pyrimido[5,4-e][1,2,4]triazine-5,7(6H,8H)-dione | C5 H3 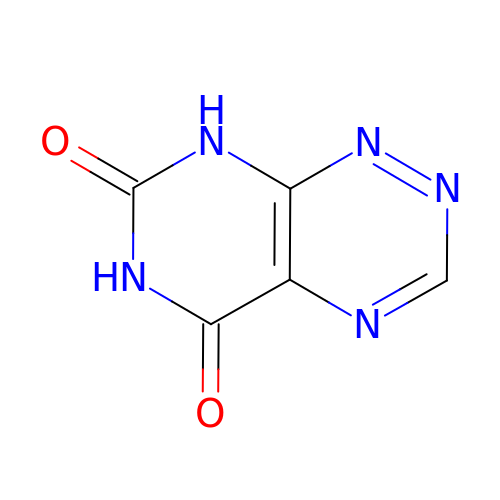N5 O2 | IDJLTUNWTSUIHO-UHFFFAOYSA-N METHYL 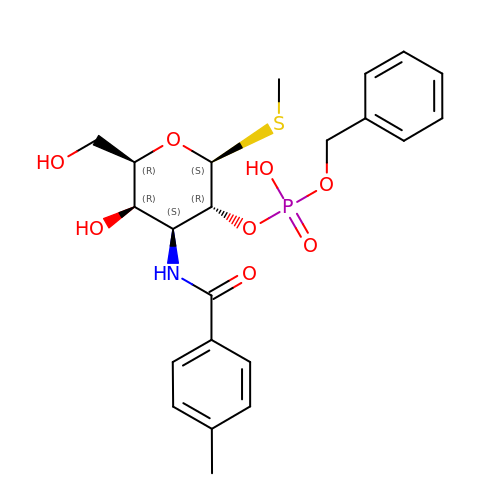2-O-[(S)-(BENZYLOXY)(HYDROXY)PHOSPHORYL]-3-DEOXY-3-{[(4-METHYLPHENYL)CARBONYL]AMINO}-1-THIO-BETA-D-GALACTOPYRANOSIDE | C22 H28 N O8 P S | IDAWZVIHHBVHNS-QWPXSNKBSA-N> MTSATASFATRTSLAADLAALGLAWGDAIMVHAAVSRVGRLLDGPDTIIAALRDTVGPGGTVLAYADWEARYEDLVDDAGRVPPEWREHVPPFDPQRSRAIRDNGVLPEFLRTTPGTLRSGNPGASLVALGAKAEWFTADHPLDYGYGEGSPLAKLVEAGGKVLMLGAPLDTLTLLHHAEHLADIPGKRIKRIEVPFATPTGTQWRMIEEFDTGDPIVAGLAEDYFAGIVTEFLAS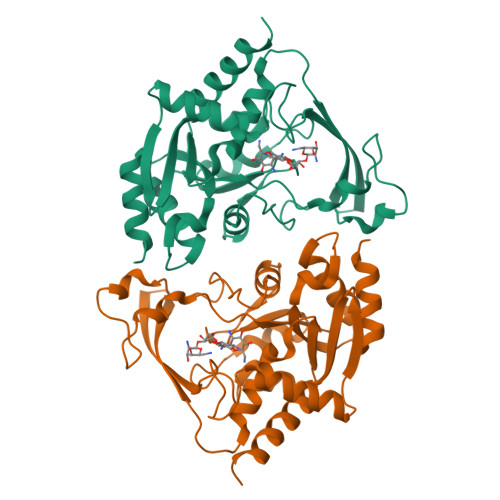GQGRQGLIGAAPSVLVDAAAITAFGVTWLEKRFGTPSP O-[2-(1,3-dioxo-1,3-dihydro-2H-isoindol-2-yl)ethyl] (4-iodophenyl)thiocarbamate | C17 H13 I N2 O3 S | 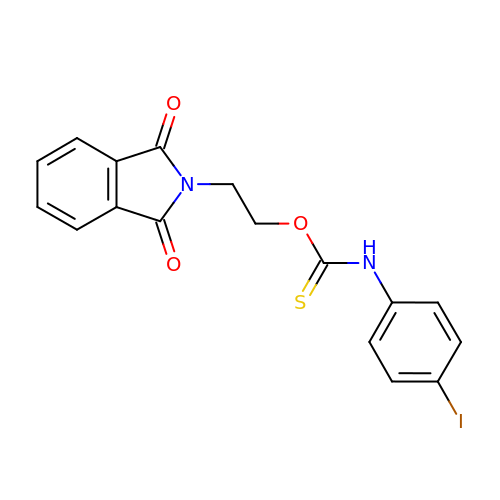CYYIBMGIJWXZEP-UHFFFAOYSA-N>MPMTVITLKNVPQSLRGDLTRWMQEIATGVYVGNFNSRIREYLWRRVQETMGAGEASMCFAARNELGYDFLTENASRSVIDYDGLPLIFIPKEQSAVSDLPKGFSTAAKLHRAHIAGSGKKKEKPIRYVVIDIETDGKDAKRNHILEIGAIRCEDGKETHFTALISGDAVPPSITKLTGITATLLQKEGQEEKKVLTAFREFIGDDDLVGYHVSFDIEFLRQAFKKYGLGYLKNKTHDLLRIVKKEQLFQADYKLETSLQSYGIHKKVPHRALGDAELVKCLAKKLNKF[2x];>MAGPIIAGKSESSELPRVEDRATFIYIEHAKINRVDSAVTVAEAKGVVRIPAAMIGVLLLGPGTDISHRAVELLGDTGTALVWVGEQGVRYYASGRALARSTRFLVKQAELVTNERSRLRVARRMYQMRFPTEDVSKLTMQQLRSHEGARVRRKYRELSKKYNVPWKKRVYNPDDFAGGDPINQALSAAHVALYGLVHSVVAALGLSPGLGFVHTGHDRSFIYDVADLYKAEITVPIAFAVAAEAEEGQDIGQLARLRTRDAFVDGKILKRMVKDLQTLLEIPEEGQIEAEPLSLWDDKEKLVPYGVNYSEVTSCP[4x]

CRISPR–Cas adaptive immune systems capture DNA fragments from invading mobile genetic elements and integrate them into the host genome to provide a template for RNA-guided immunity. Here we reconstitute CRISPR sequence capture, processing and integration by a naturally occurring Megasphaera NM10-related Cas2 and DEDDh fusion protein (Cas2/DEDDh) in complex with Cas1 (Cas1–Cas2/DEDDh). The natural Cas1–Cas2/exonuclease fusion (trimmer-integrase) catalyses coordinated DNA capture, trimming and integration. The Megasphaera Cas1–Cas2 retains the canonical heterohexameric architecture, with two Cas1 dimers (denoted Cas1 and Cas1′, a or b subunit) bridged by a central Cas2 dimer.

Cryo-EM was used to solve 3.1 Å and 2.9 Å resolution structures of Cas1–Cas2/DEDDh complexed with prespacer substrates with and without a TT PAM, respectively. A 23 bp duplex sits on the top of the complex, while 5-nucleotide single-stranded 3′ overhangs extend into the clefts formed at opposite Cas1 interfaces. The DEDDh domain could not be resolved in the PAM-absent dataset, presumably due to a high degree of conformational flexibility conferred by the 38 amino acid linker between DEDDh and Cas2, and because all 3′ ends are buried within the complex, protected from exonuclease activity. Dual Cas1 His29 histidyl residues measure out a 23 bp DNA duplex by π-stacking with the terminal base pairs of the double-stranded region, clasping the prespacer strands and marking the start of the single-stranded 3′ overhang. In the absence of a TT PAM, DEDDh trims prespacer strands to the integration-competent size (28 nucleotides). When the PAM is absent, the substrates are fully trimmed, underscoring the necessity of sequence-specific interactions for asymmetric trimming and PAM protection. Loop 7, helix 7 and the C-terminal cap are absent in the PAM-deficient density, suggesting that these structural motifs participate in PAM protection.> 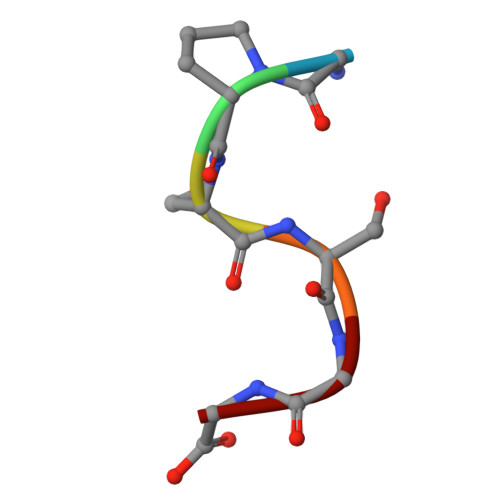GPSSGG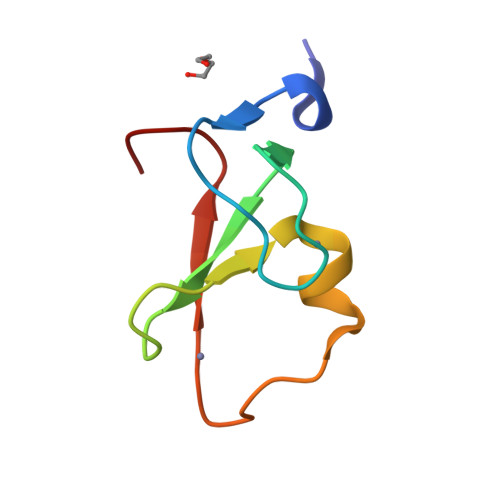>[2x]SDQEAKIHPGVTCDGCQMFPINGSRFKCRNCDDFDFCETCFKTKKHNTRHTFGRINEPGQ> V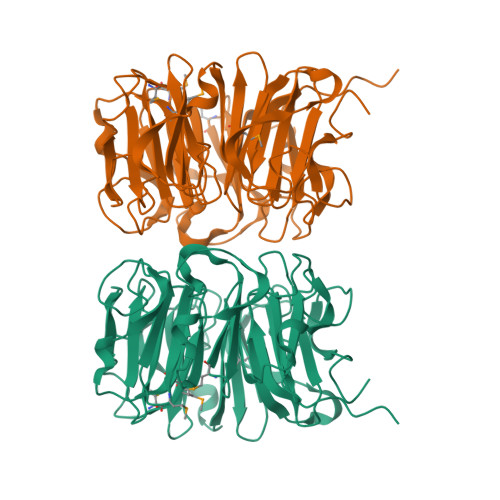TAPPRKVLIISAGASHSVALLSGDIVCSWGRGEDGQLGHGDAEDRPSPTQLSALDGHQIVSVTCGADHTVAYSQSGMEVYSWGWGDFGRLGHGNSSDLFTPLPIKALHGIRIKQIACGDSHCLAVTMEGEVQSWGRNQNGQLGLGDTEDSLVPQKIQAFEGIRIKMVAAGAEHTAAVTEDGDLYGWGWGRYGNLGLGDRTDRLVPERVTSTGGEKMSMVACGWRHTISVSYSGALYTYGWSKYGQLGHGDLEDHLIPHKLEALSNSFISQISGGARHTMALTSDGKLYGWGWNKFGQVGVGNNLDQCSPVQVRFPDDQKVVQVSCGWRHTLAVTERNNVFAWGRGTNGQLGIGESVDRNFPKIIEALSVDG>EFRDCAEVFKSGHTTNGIYTLTFPNSTEEIKAYCDMEAGGGGWTIIQRREDGSVDFQRTWKEYKVGFGNPSGEYWLGNEFVSQLTNQQRYVLKIHLKDWEGNEAYSLYEHFYLSSEELNYRIHLKGLTGTAG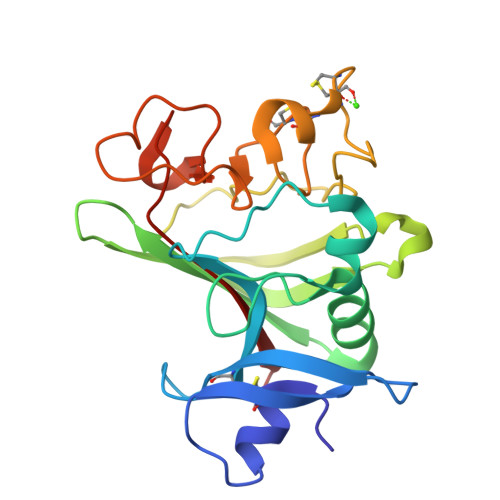KISSISQPGNDFSTKDGDNDKCICKCSQMLTGGWWFDACGPSNLNGMYYPQRQNTNKFNGIKWYYWKGSGYSLKATTMMIRPADF[2x]> MSGFSPELIDYL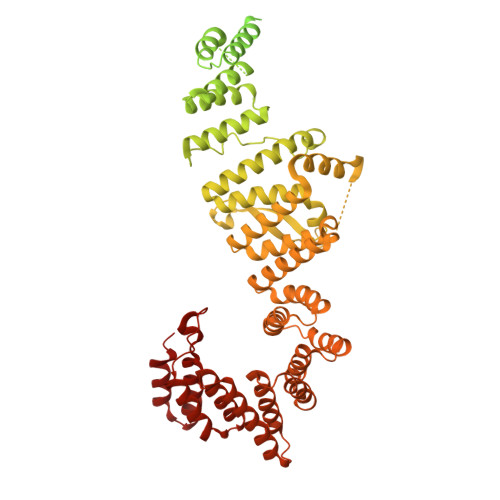EGKISFEEFERRREERKTREKKSLQEKGKLSAEENPDDSEVPSSSGINSTKSQDKDVNEGETSDGVRKSVHKVFASMLGENEDDEEEEEEEEEEEEEEETPEQPTAGDVFVLEMVLNRETKKMMKEKRPRSKLPRALRGLMGEANIRFARGEREEAILMCMEIIRQAPLAYEPFSTLAMIYEDQGDMEKSLQFELIAAHLNPSDTEEWVRLAEMSLEQDNIKQAIFCYTKALKYEPTNVRYLWERSSLYEQMGDHKMAMDGYRRILNLLSPSDGERFMQLARDMAKSYYEANDVTSAINIIDEAFSKHQGLVSMEDVNIAAELYISNKQYDKALEIITDFSGIVLEKKTSEEGTSEENKAPENVTCTIPDGVPIDITVKLMVCLVHLNILEPLNPLLTTLVEQNPEDMGDLYLDVAEAFLDVGEYNSALPLLSALVCSERYNLAVVWLRHAECLKALGYMERAAESYGKVVDLAPLHLDARISLSTLQQQLGQPEKALEALEPMYDPDTLAQDANAAQQELKLLLHRSTLLFSQGKMYGYVDTLLTMLAMLLKVAMNRAQVCLISSSKSGERHLYLIKVSRDKISDSNDQESANCDAKAIFAVLTSVLTKDDWWNLLLKAIYSLCDLSRFQEAELLVDSSLEYYSFYDDRQKRKELEYFGLSAAILDKNFRKAYNYIRIMVMENVNKPQLWNIFNQVTMHSQDVRHHRFCLRLMLKNPENHALCVLNGHNAFVSGSFKHALGQYVQAFRTHPDEPLYSFCIGLTFIHMASQKYVLRRHALIVQGFSFLNRYLSLRGPCQESFYNLGRGLHQLGLIHLAIHYYQKALELPPLVVEGIELDQLDLRRDIAYNLSLIYQSSGNTGMAQTLLYTYCSI> MFRMPRPIRATALSAAVLAGALASTPAQATVGDPTTDAKLDFTARLTIGTDYRSCSGALVDTQWVLTAASCFADDPNQPDTVAAGKPAQLTRATVGRADSNIANGYVREVVELVPHPERDMVLARLDKAIPDIAPVRLASDAPTAGTPLTAVGFGRTKDEWVPIQRHQGAFTVTSVTAGAVNVTGQGGDAICAGDTGGPLLQDKNGTLHLVGVNNRSMQGGCYGSETTSTDAIAAMSDADFVTQTVNRDLGTGNLSDLVASADFNSDGRTDVAAVLEDGSLHAFYAKPDGTLEYGRELWNDNTWSPMVQIIGGDFNSDGNGDIAAVRSDGTLNLYTGTATGILNK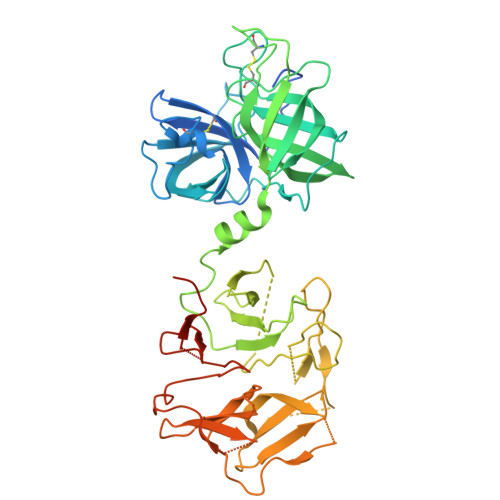SKPMWHDTSWKTIKQVTRFKFNGRDGLVAQWGDGNLYGYYTGTDGTLTGTKVKMWPDATWGKTRLTGTADINADGRDDLTAVRDDGSLNWYAGNTKGGLDAARKLWPDNTWTPMKRIIGGDFNGDNKGDIAAVGGQSTLLLYTGTGTGTLNKGIAMRPASGSHHHHHHHH>GSHMVHRKLIIDTDCGGDDAIAIMLAMTQPDVEVIAITVVWGNVEVNQGMENIGKLLDLYDADIPFFRGAEGPLVGERETVQWGGFGSDGFGDAGFPPSQRVALQPKRHAALEILKILEEAEPSDDVVYQLVALGPLTNVALALRLNPDLFSKLGTDTIPGIVIMNGTSESKGNSNMAAEFNSHCDPEAGVVVLQHKGWKCPVQLVNWEVTVNSPM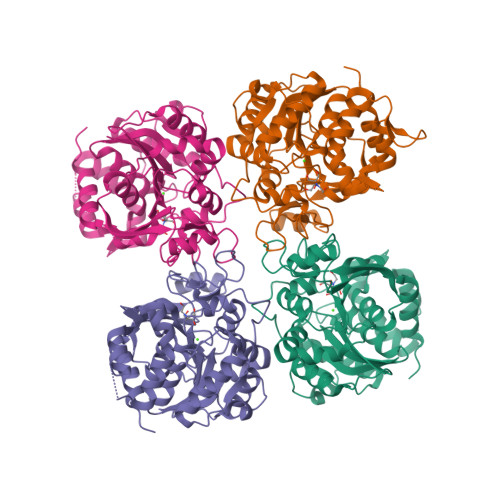TWGFYDKLVNRESTPNGRVAVNQNKWQEFIEKLFQRLEAFTRIHDDGTRADTGDAEATQDVTCVVPDAVAVLVAIRPESVLDSFLTYVTVELHGRETRGATCIDWYGTEQSMAKKGRWRNCNVITKVDNEMFLKALRDIVEYVA[4x]>[2x]PVIQCDIRQGRTAEQKQAMAEAITRAVHET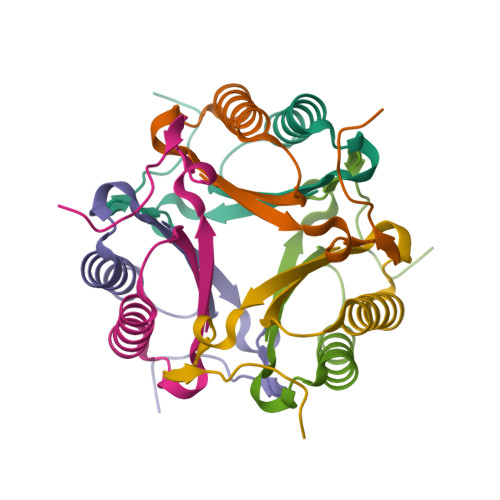IGAPVEYIYVLIRETPGAHHVKAGRTLPEYTGDG>MGFSADHSQIAQTKDTMFTGYLDPVQAKDYFAEAEKTSIVQRVAQKIPMGATGIVIPHWTGDVSAQWIGEGDMKPITKGNMTKRDVHPAKIATIFVASAETVRANPANYLGTMRTKVATAIAMAFDNAALHGTNAPSAFQGYLDQSNKTQSISPNAYQGLGVSGLTKLVTDGKKWTHTLLDDTVEPVLNGSVDANGRPLFVESTYESLTTPFREGRILGRPTILSDHVAEGDVVGYAGDFSQIIWGQVGGLSFDVTDQATLNLGSQESPNFVSLWQHNLVAVRVEAEYGLLINDVNAFVKLTFDPVLTTYALDLDGASAGNFTLSLDGKTSANIAYNASTATVKSAIVAIDDGVSADDVTVTGSAGDYTITVPGTLTADFSGLTDGEGASISVVSVG[30x];>[12x]MAETESIDPEKLRDQLLDAFENKQNELKSSKAYYDAERRPDAIGLAVPLDMRKYLAHVGYPRTYVDAIAERQELEGFRIPSANGEEPESGGENDPASELWDWWQANNLDIEATLGHTDALIYGTAYITISMPDPEVDFDVDPEVPLIRVEPPTALYAEVDPRTRKVLYAIRAIYGADGNEIVSATLYLPDTTMTWLRAEGEWEAPTSTPHGLEMVPVIPISNRTRLSDLYGTSEISPELRSVTDAAAQILMNMQGTANLMAIPQRLIFGAKPEELGIN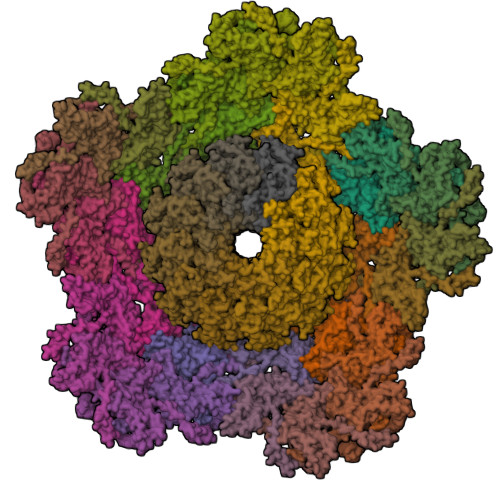AETGQRMFDAYMARILAFEGGEGAHAEQFSAAELRNFVDALDALDRKAASYSGLPPQYLSSSSDNPASAEAIKAAESRLVKKVERKNKIFGGAWEQAMRLAYKMVKGGDIPTEYYRMETVWRDPSTPTYAAKADAAAKLFANGAGLIPRERGWVDMGYTIVEREQMRQWLEQDQKQGLGLIGSLYGASTPEGKPGEAPVGEPPAPEPDAA>[2x]MARFNAAFTRIKIMFSRIRGLISCQSNTQTIAPTLSPPSSGHVSFAGIDYPLLPLNHQTPLVFQWFERNPDRFGQNEIPIINTQKNPYLNNIINAAIIEKERIIGIFVDGDFSKGQRKALGKLEQNYRNIKVIYNSDLNYSMYDKKLTTIYLENITKLEAQSASERDEVLLNGVKKSLEDVLKNNPEETLISSHNKDKGH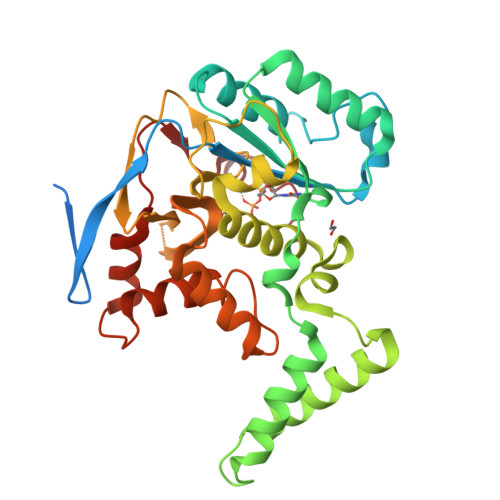LWFDFYRNLFLLKGSDAFLEAGKPGCHHLQPGGGCIYLDADMLLTDKLGTLYLPDGIAIHVSRKDNHVSLENGIIAVNRSEHPALIKGLEIMHSKPYGDPYNDWLSKGLRHYFDGSHIQDYDAFCDFIEFKHENIIMNTSSLTASSWR>[3x]NSTNIKWHECSVEKVDRQRLLDQKGCVIWVTGLSGSGK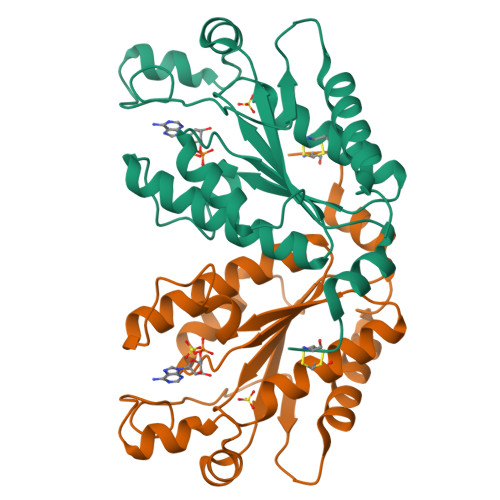STLACALNQMLYQKGKLCYILDGDNVRHGLNRDLSFKAEDRAENIRRVGEVAKLFADAGIICIASLISPYRTDRDACRSLLPEGDFVEVFMDVPLSVCEARDPKGLYKLARAGKIKGFTGIDDPYEPPLNCEISLGREGGTSPIEMAEKVVGYLDNKGYLQA2-[1-(4-hydroxyphenyl)-1H-1,2,3-triazol-4-yl]-7-methyl-1,7-naphthyridin-8(7H)-one 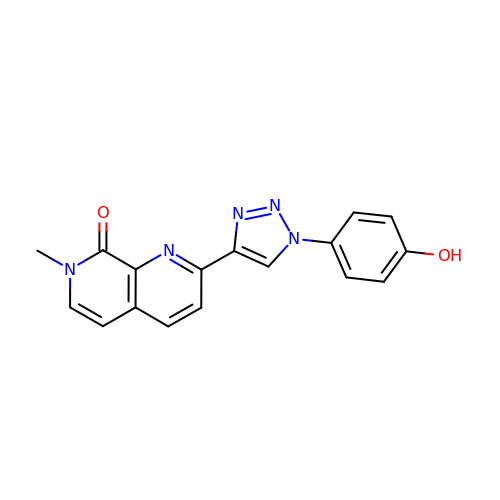| C17 H13 N5 O2 | KANBQBQJUNGFMT-UHFFFAOYSA-N> SMAENEIEEMLEHLRRIKSGGDLDWLDILRIEELEM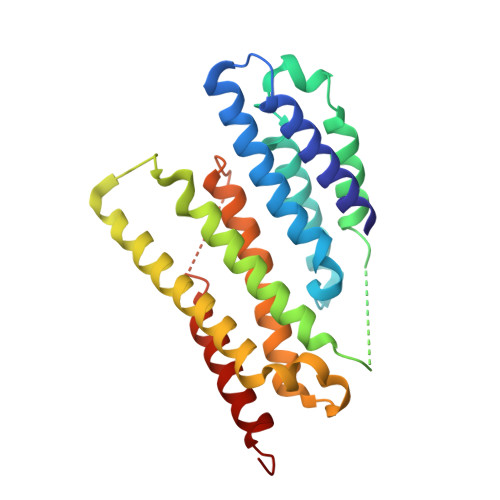VLRVFRTFTKYNDVLLPDSLVELTKRAKLIGEILHRLFGRIPHKCKTNLNLERLESHLLEFFQGNTASLSHNYELNNFDLSKYMDCLENFLNDVLMMFLQKDRFFHSREQLAKHRSIKELKIVQKKIRFLKYIYATEINGYVDYEKQECLENRIQFMTNTVGQYCLAVLDYVTEGKLNEENDNFSKPPYLLSLIVLVELEMKKIFHGEVK>GSSMDNQDGFILQQVKLSLDDPDSYLSSWNSNDASPCRWSGVSCAGDFSSVTSVDLSSANLAGPFPSVICRLSNLAHLSLYNNSINSTLPLNIAACKSLQTLDLSQNLLTGELPQTLADIPTLVHLDLTGNNFSGDIPASFGKFENLEVLSLVYNLLDGTIPPFLGNISTLKMLNLSYNPFSPSRIPPEFGNLTNLEVMWLTECHLVGQIPDSLGQLSKLVDLDLALNDLVGHIPPSLGGLTNVVQIELYNNSLTGEIPPELGNLKSLRLLDASMNQLTGKIPDELCRVPLESLNLYENNLEGELPASIALSPNLYEIRIFGNRLTGGLPKDLGLNSPLRWLDVSENEFSGDLPADLCAKGELEELLIIHNSFSGVIPESLADCRSLTRIRLAYNRFSGSVPTGFWGLPHVNLLELVNNSFSGEISKSIGGASNLSLLILSNNEFTGSLPEEIGSLDNLNQLSASGNKFSGSLPDSLMSLGELGTLDLHGNQFSGELTSGIKSWKKLNELNLADNEFTGKIPDEIGSLSVLNYLDLSGNMFSGKIPVSLQSLKLNQLNLSYNRLSGDLPPSLAKDMYKNSFIGNPGLCGDIKGLCGSENEAKKRGYVLEGSENLYFQ[2x];>[2x]GSSMASANLEGDALHTLRVTLVDPNNVLQSWDPTLVNPCTWFHVTCNNENSVIRVDLGNAELSGHLVPELGVLKNLQYLELYSNNITGPIPSNLGNLTNLVSLDLYLNSFSGPIPESLGKLSKLRFLRLNNNSLTGSIPMSLTNITTLQVLDLSNNRLSGSVPDNGSFSLFTPISFANNLDLCGPVTSHPCPGSLENLYFQ;>PVPTSGPSRKHN[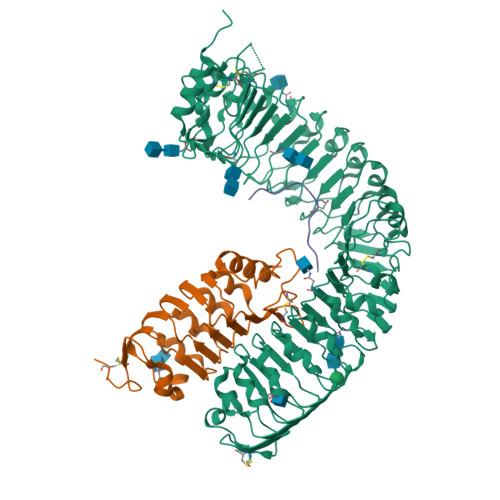2x]> MDLTNGGVSPAATSAPLDWTTFRRVFLIDDAWRPLMEPELANPLTAHLLAEYNRRCQTEEVLPPREDVFSWTRYCTPDEVRVVIIGQNPYHHPGQAHGLAFSVRANVPPPPSLRNVLAAVKNCYPEARMSGHGCLEKWARDGVLLLNTTLTVKRGAAASHSRIGWDRFVGGVIRRLAARRPGLV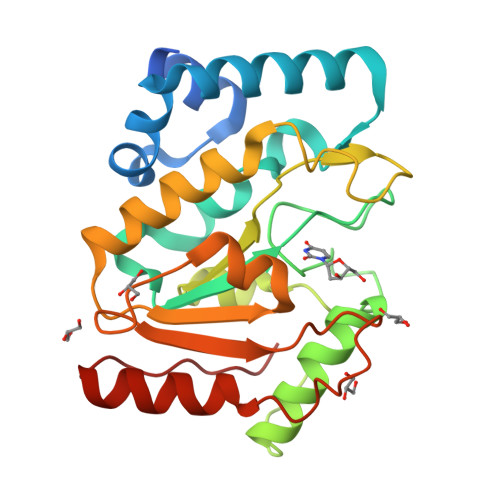FMLWGTHAQNAIRPDPRVHCVLKFSNPSPLSKVPFGTCQHFLVANRYLETRSISPIDWSV> DRHHHHHHKLKDIRHSSDDDLLLPYTKSHGPSHSHRYVRDCQPVAHGTVTHETQAASKHSNSPVLESNIFISDITDDSGTHRWVSGHITEVHDPLRSVSVLEPGGPGGCAHNHRELVEVTAKTRKCLVAQNGGYFDTHTGQCLGNIISDGKLVRNSGGIQNAQFGIRKDGTLVFGYLSEDDILDQENPFVQLISGVVWLLRKGE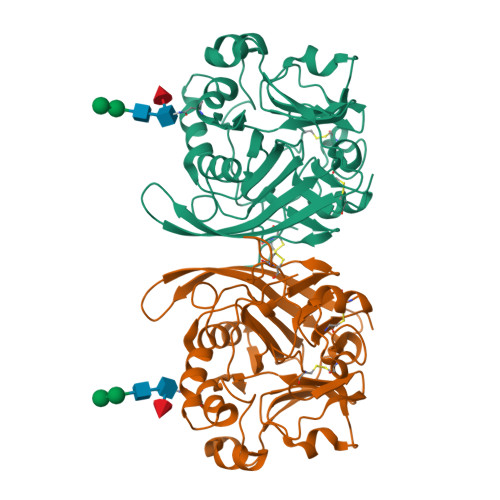IYINESIQAECDKTQETGNFRHFVDVISARTAVGHDKEGKLILFHVDGQTDVRGMNLWQVAKFLKDQNVMNAINLDGGGSATYVLNGSLASYPSDHCNPSKWRCPRAISTVLCIHER>[8x]MAQRMTTQLLLLLVWVAVVGEAQTRIAWARTELLNVCMNAKHHKEKPGPEDKLHEQCRPWRKNACCSTNTSQEAHKDVSYLYRF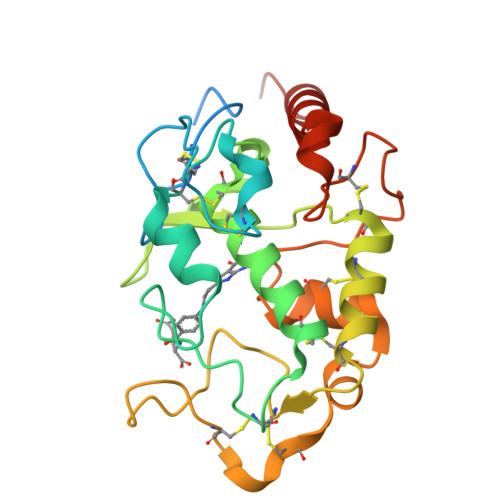NWNHCGEMAPACKRHFIQDTCLYECSPNLGPWIQQVDQSWRKERVLNVPLCKEDCEQWWEDCRTSYTCKSNWHKGWNWTSGFNKCAVGAACQPFHFYFPTPTVLCNEIWTHSYKVSNYSRGSGRCIQMWFDPAQGNPNEEVARFYAAAMSGTLV>AAATATTT[1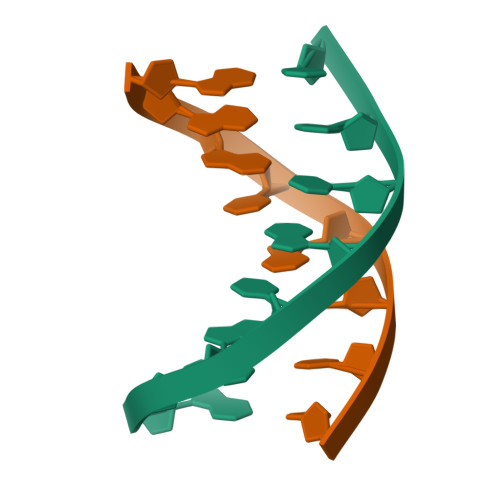1x]>[2x]AGIHHHHHHSSEPSCRFAHQYTQEQVLQNPSKFINDVLFWEGKFHQNNISYNSGNGMSYDGTNIDWVTGEGTVKHPFSAASKESLQVMLYAHAIAGSADAARFLSPNNPSAAPGIAASIMDTKLQTYLRFNETYPGFGGFLPWFTSSSQDLTPTWDWNNRVPGLDNGELLWAVYAFIQAAENTSNK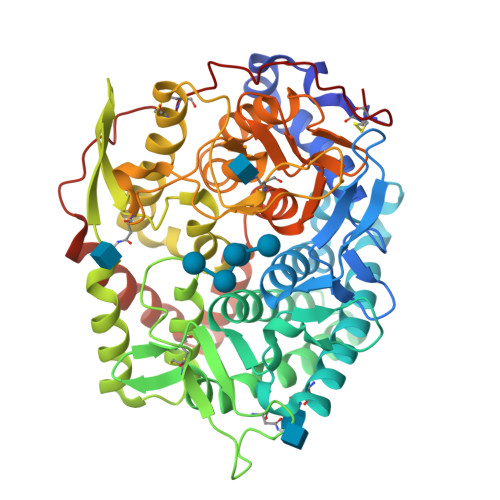SFIDLAKKWQTWMDYTKTTAAHIFYQGEGKVCAVTDIKNQSLPVYHPEQTYACEGTSYLNDPYQGELFTWWLQFFGGLSDADIEALWEYKRPQLVSVDYHIGNVGPITVQKGYWFSSHETWKVLEMPYYDIDIIRRVFQNAERARTCNSVVTQVPGMFASINNVTDPATGDVVGYISNAGIPSIANQTIQELDVITPYSVFPTVLFDKGVGMAWWRNMAIGKKMQNIYGSTESTRRDGTGVSALLTWDSKVSTVNAILGGVSGLVSQKMKAENIYNTFVERIEAEYSRVFKNLKGEHVPFCLPQETVPDTGLVDFTTCN(2E)-2-{[(2S)-2-(ACETYLAMINO)-2-CARBOXYETHOXY]IMINO}PENTANEDIOIC 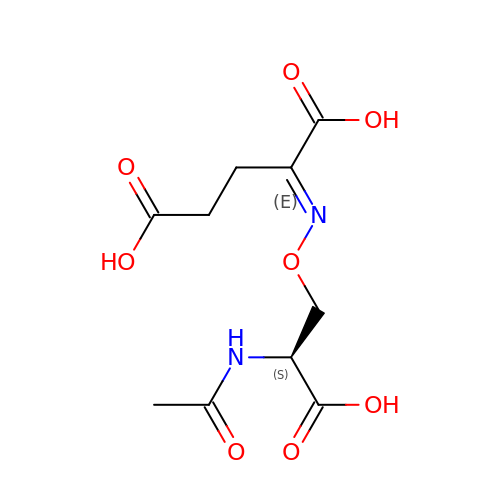ACID | C10 H14 N2 O8 | ULEFFWARYSNNRF-NYYVKIQXSA-N>GHMKETYTPEEYLKNYALSVCIAEGYSAKEVKNDAAAAARGYTEFGDYSLEAHTAVRALAKEFLA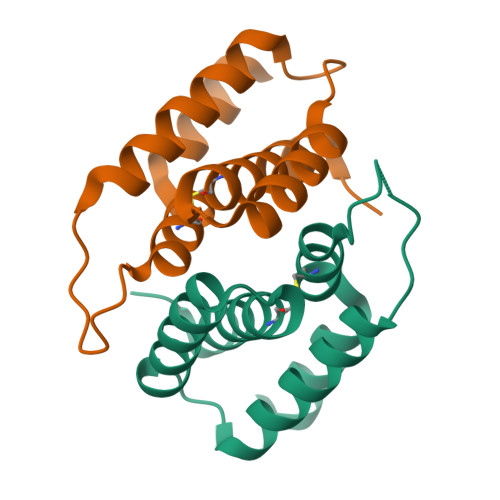KPYDSMSGEPMTMAKCIDLVHSQELQAIIKKYQGKDDN[4x]> MAGSREILLPEVHLNSPIVKHKLYYYILLGNLPNEIDLDDLGPLHNQNWNQIAHEESNLAQRLVNVRNFLITHIPDLRKGHWQEYVNVILWPRILPLIPDFKINDQLPLLKNWDKLVKESCSVINAGTSQCIQNLSYGLTGRGNLFTRSRELSGDRRDIDLKTVVAAWHDSDWKRISDFWIMIKFQMRQLIVRQTDHNDSDLITYIENREGIIIITPELVALFNTENHTLTYMTFEIVLMVSDMYEGRHNILSLCTVSTYLNPLKKRITYLLSLVDNLAFQIGDAVYNIIALLESFVYAQLQMSDPIPELRGQFHAFVCSEILDALRGTNSFTQDELRTVTTNLISPFQDLTPDLTAELLCIMRLWGHPMLTASQAAGKVRESMCAGKVLDFPTIMKTLAFFHTILINGYRRKHHGVWPPLNLPGNASKGLTELMNDNTEISYEFTLKHWKEVSLIKFKKCFDADAGEELSIFMKDKAISAPKQDWMSVFRRSLIKQRHQHHQVPLPNPFNRRLLLNFLGDDKFDPNVELQYVTSGEYLHDDTFCASYSLKEKEIKPDGRIFAKLTKRMRSCQVIAESLLANHAGKLMKENGVVMNQLSLTKSLLTMSQIGIISEKARKSTRDNINQPGFQNIQRNKSHHSKQVNQRDPSDDFELAASFLTTDLKKYCLQWRYQTIIPFAQSLNRMYGYPHLFEWIHLRLMRSTLYVGDPFNPPADTSQFDLDKVINGDIFIVSPRGGIEGLCQKAWTMISIAVIILSATESGTRVMSMVQGDNQAIAVTTRVPRSLPTLEKKTIAFRSCNLFFERLKCNNFGLGHHLKEQETIISSHFFVYSKRIFYQGRILTQALKNASKLCLTADVLGECTQSSCSNLATTVMRLTENGVEKDICFYLNIYMTIKQLSYDIIFPQVSIPGDQITLEYINNPHLVSRLALLPSQLGGLNYLSCSRLFNRNIGDPVVSAVADLKRLIKSGCMDYWILYNLLGRKPGNGSWATLAADPYSINIEYQYPPTTALKRHTQQALMELSTNPMLRGIFSDNAQAEENNLARFLLDREVIFPRVAHIIIEQTSVGRRKQIQGYLDSTRSIMRKSLEIKPLSNRKLNEILDYNINYLAYNLALLKNAIEPPTYLKAMTLETCSIDIARNLRKLSWAPLLGGRNLEGLETPDPIEITAGALIVGSGYCEQCAAGDNRFTWFFLPSGIEIGGDPRDNPPIRVPYIGSRTDERRVASMAYIRGASSSLKAVLRLAGVYIWAFGDTLENWIDALDLSHTRVNITLEQLQSLTPLPTSANLTHRLDDGTTTLKFTPASSYTFSSFTHISNDEQYLTINDKTADSNIIYQQLMITGLGILETWNNPPINRTFEESTLHLHTGASCCVRPVDSCILSEALTVKPHITVPYSNKFVFDEDPLSEYETAKLESLSFQAQLGNIDAVDMTGKLTLLSQFTARQIINAITGLDESVSLTNDAIVASDYVSNWISECMYTKLDELFMYCGWELLLELSYQMYYLRVVGWSNIVDYSYMILRRIPGAALNNLASTLSHPKLFRRAINLDIVAPLNAPHFASLDYIKMSVDAILWGCKRVINVLSNGGDLELVVTSEDSLILSDRSMNLIARKLTLLSLIHHNGLELPKIKGFSPDEKCFALTEFLRKVVNSGLSSIENLSNFMYNVENPRLAAFASNNYYLTRKLLNSIRDTESGQVAVTSYYESLEYIDSLKLTPHVPGTSCIEDDSLCTNDYIIWIIESNANLEKYPIPNSPEDDSNFHNFKLNAPSHHTLRPLGLSSTAWYKGISCCRYLERLKLPQGDHLYIAEGSGASMTIIEYLFPGRKIYYNSLFSSGDNPPQRNYAPMPTQFIESVPYKLWQAHTDQYPEIFEDFIPLWNGNAAMTDIGMTACVEFIINRVGPRTCSLVHVDLESSASLNQQCLSKPIINAIITATTVLCPHGVLILKYSWLPFTRFSTLITFLWCYFERITVLRSTYSDPANHEVYLICILANNFAFQTVSQATGMAMTLTDQGFTLISPERINQYWDGHLKQERIVAEAIDKVVLGENALFNSSDNELILKCGGTPNARNLIDIEPVATFIEFEQLICTMLTTHLKEIIDITRSGTQDYESLLLTPYNLGLLGKISTIVRLLTERILNHTIRNWLILPPSLRMIVKQDLEFGIFRITSILNSDRFLKLSPNRKYLIAQLTAGYIRKLIEGDCNIDLTRPIQKQIWKALGCVVYCHDPMDQRESTEFIDININEEIDRGIDGEEI;>MDPTDLSFSPDEINKLIETGLNTVEYFTSQQVTGTSSLGKNTIPPGVTGLLTNAAEAKIQESTNHQKGSVGGGAKPKKPRPKIAIVPADDKTVPGKPIPNPLLGLDSTPSTQTVLDLSGKTLPSGSYKGVKLAKFGKENLMTRFIEEPRENPIATSSPIDFKRGAGIPAGSIEGSTQSDGWEMKSRSLSGAIHPVLQSPLQQGDLNALVTSVQSLALNVNEILNTVRNLDSRMNQLETKVDRILSSQSLIQTIKNDIVG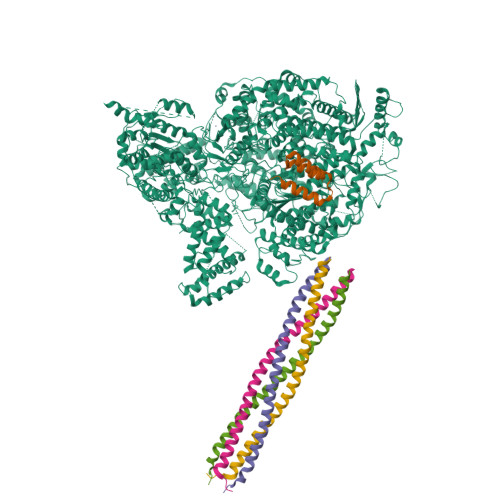LKAGMATLEGMITTVKIMDPGVPSNVTVEDVRKTLSNHAVVVPESFNDSFLTQSEDVISLDELARPTATSVKKIVRKVPPQKDLTGLKITLEQLAKDCISKPKMREEYLLKINQASSEAQLIDLKKAIIRSAI[5x]>MHIDNIENLSDREFDYIVVGGGSAGAAVAARLSEDPAVSVALVEAGPDDRGVPEVLQLDRWMELLESGYDWDYPIEPQENGNSFMRHARAKVMGGCSSHNSCIAFWAPREDLDEWEAKYGATGWNAEAAWPLYKRLETNEDAGPDAPHHGDSGPVHLMNVPPKDPTGVALLDACEQAGIPRAKFNTGTTVVNGANFFQINRRADGTRSSSSVSYIHPIVEQENFTLLTGLRARQLVFDADRRCTGVDIVDSAFGHTHRLTARNEVVLSTGAIDTPKLLMLSGIGPAAHLAEHGIEVLVDSPGVGEHLQDHPEGVVQFEAKQPMVAEST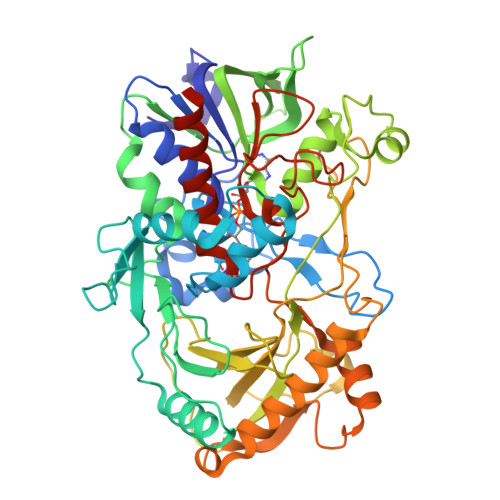QWWEIGIFTPTEDGLDRPDLMMHYGSVPFDMNTLRHGYPTTENGFSLTPNVTHARSRGTVRLRSRDFRDKPMVDPRYFTDPEGHDMRVMVAGIRKAREIAAQPAMAEWTGRELSPGVEAQTDEELQDYIRKTHNTAYHPVGTVRMGAVEDEMSPLDPELRVKGVTGLRVADASVMPEHVTVNPNITVMMIGERCADLIRSARAGETTTADAELSAALA[2x]>MQIPASEQETLVRPKPLLLKLLKSVGAQKDTYTMKEVLFYLGQYIMTKRLYDEKQQHIVYCSNDLLGDLFGVPSFSVKEHRKIYTMIYRNLVVVNQQESSDSGTSV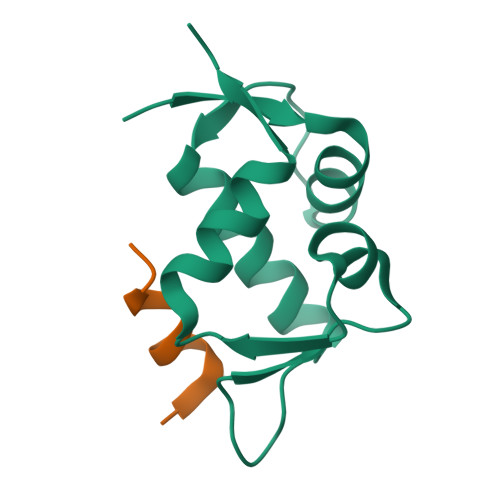SEN[2x];>[2x]LTFEHYWAQLTS>MPQFASKAEEKNYYERQASLAEFLTWYHQQELPEYEKPSLTVDMVLLCYNKEADQLKVLLIQRKGHPFRNSWALPGGFVNRNESTEDSVLRETKEETGVVISQENIEQLHSFSRPDRDPRGWVVTVSYLAFIGEEPLIAGDDAKEVHWFNLERHGQHITLSHEDVEITLDLKTAASL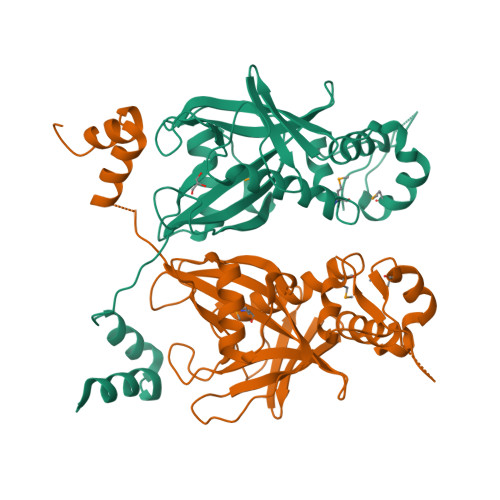GKDTLAFDHSEIIIKAFNRVVDKMEHEPQVLQVLGKDFTITEARKVFAKFLGVDYRSIDHSNFKKAMTQYFEELGERPVGIGRPSKIYQLKTTTGF[2x]> GHMAKQYDSVECPFCDEVSKYEKLAKIGQGTFGE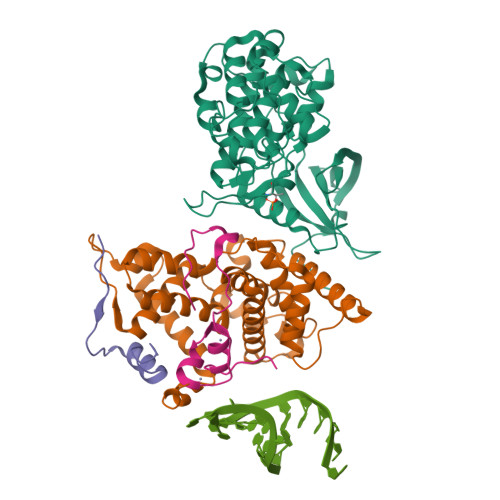VFKARHRKTGQKVALKKVLMENEKEGFPITALREIKILQLLKHENVVNLIEICRTKASPYNRCKGSIYLVFDFCEHDLAGLLSNVLVKFTLSEIKRVMQMLLNGLYYIHRNKILHRDMKAANVLITRDGVLKLADFGLARAFSLAKNSQPNRYTNRVVTLWYRPPELLLGERDYGPPIDLWGAGCIMAEMWTRSPIMQGNTEQHQLALISQLCGSITPEVWPNVDNYELYEKLELVKGQKRKVKDRLKAYVRDPYALDLIDKLLVLDPAQRIDSDDALNHDFFWSDPMPSDLKGMLST;> MEGERKNNNKRWYFTREQLENSPSRRFGVDPDKELSYRQQAANLLQDMGQRLNVSQLTINTAIVYMHRFYMIQSFTQFPGNSVAPAALFLAAKVEEQPKKLEHVIKVAHTCLHPQESLPDTRSEAYLQQVQDLVILESIILQTLGFELTIDHPHTHVVKCTQLVRASKDLAQTSYFMATNSLHLTTFSLQYTPPVVACVCIHLACKWSNWEIPVSTDGKHWWEYVDATVTLELLDELTHEFLQILEKTPNRLKRIWNWRACEAA;> SPLFAEPYKVTSKEDYLSSRIQSMLGNYDEMKDFIG;> XMEPVDPRLEPWKHPGSQPKTACTNCYCKKCCFHCQVCFITKALGISYGRKKRRQRRR> SMRKTIERLLNSELSSNSIAVRTGVSQAVISKLRNGKKELGNLTLNSAEKLFEYQKEMEKVDTWIVYRGRTADMNKSYIAEGSTYEEVYNNFVDKYGYDVLDEDIYEIQLLKKNGENLDDYDVDSDGINNYDK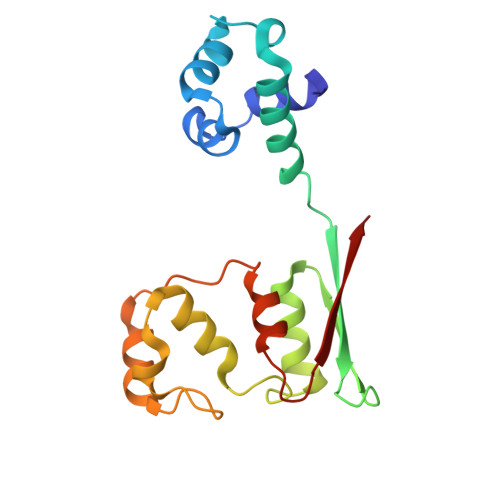LDEFRESDYVDLEDYDYRELFENSSSQVYYHEFEITHE>SNAETSDQRKAEEHIEKEAKYLASLLDAGNLNNQANEKIIKDAGGALDVSASVIDTDGKVLYGSNGRSADSQKVQALVSGHEGILSTTDNKLYYGLSLRSEGEKT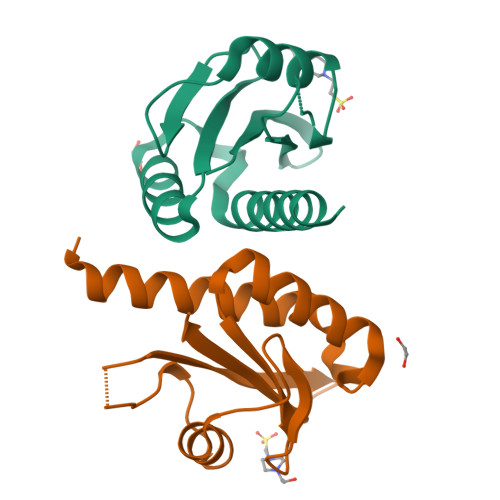GYVLLSASEKSDGLKGE[2x]> MPISPIETVPVKLKPGMDGPKVKQWPLTEEKIKALVEICTEMEKEGKISKIGPENPYNTPVFAIKKKDSTKWRKLVDFRELNKRTQDFWEVQLGIPHPAGLKKKKSVTVLDVGDAY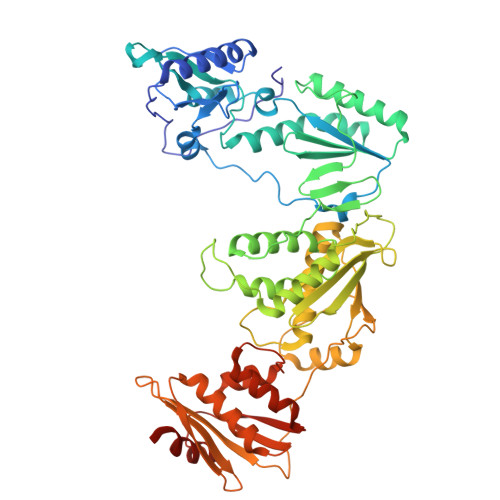FSVPLDEDFRKYTAFTIPSINNETPGIRYQYNVLPQGWKGSPAIFQSSMTKILEPFRKQNPDIVIYQYMDDLYVGSDLEIGQHRTKIEELRQHLLRWGLTTPDKKHQKEPPFLWMGYELHPDKWTVQPIVLPEKDSWTVNDIQKLVGKLNWASQIYPGIKVRQLCKLLRGTKALTEVIPLTEEAELELAENREILKEPVHGVYYDPSKDLIAEIQKQGQGQWTYQIYQEPFKNLKTGKYARMRGAHTNDVKQLTEAVQKITTESIVIWGKTPKFKLPIQKETWETWWTEYWQATWIPEWEFVNTPPLVKLWYQLEKEPIVGAETFYVDGAANRETKLGKAGYVTNRGRQKVVTLTDTTNQKTELQAIYLALQDSGLEVNIVTDSQYALGIIQAQPDQSESELVNQIIEQLIKKEKVYLAWVPAHKGIGGNEQVDKLVSAGIRKVLVPR> VTKPYSSPPTNLRSLRDRLTQVAERQGVVFGRLQRHVAMIVVAQFAATLTDDTGAPLLLVKGGSSLELRRGIPDSRTSKDFDTVARRDIELIHEQLADAGETGWEGFTAIFTAPEEIDVPGMPVKPRRFTAKLSYRGRAFATVPIEVSSVEAGNADQFDTLTSDALGLVGVPAAVAVPCMTIPWQIAQALHAVTAVLEEPKVNDRAHDLVDLQLLEGLLLDADLMPTRSACIAIFEARAQHPWPPRVATLPHWPLIYAGALEGLDHLELARTVDAAAQAV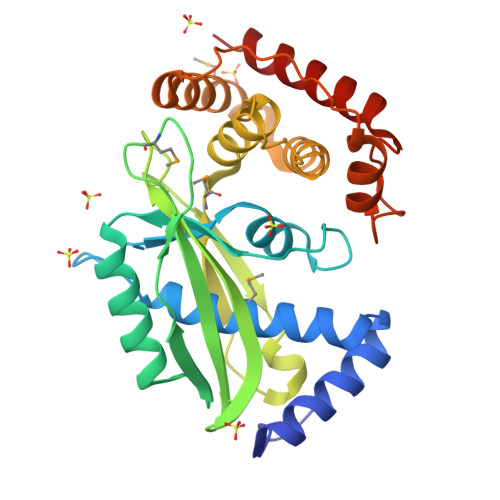QRFVARIDRATKR(2S)-1,1,1-trifluoropropan-2-yl 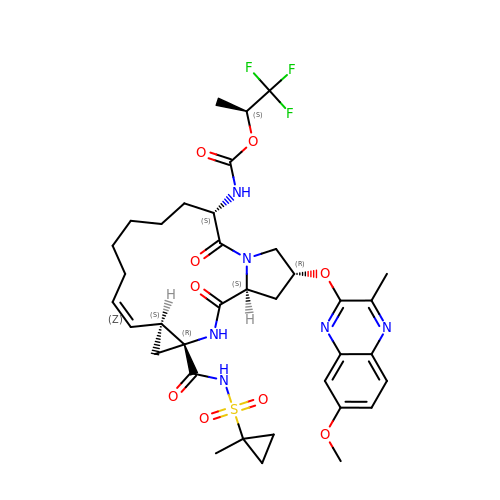{(2R,4S,6S,12Z,13aS,14aR,16aS)-2-[(7-methoxy-3-methylquinoxalin-2-yl)oxy]-14a-[(1-methylcyclopropane-1-sulfonyl)carbamoyl]-5,16-dioxo-1,2,3,5,6,7,8,9,10,11,13a,14,14a,15,16,16a-hexadecahydrocyclopropa[e]pyrrolo[1,2-a][1,4]diazacyclopentadecin-6-yl}carbamate | C36 H45 F3 N6 O9 S | RTCPQVJDZHADDP-NOIRXTOFSA-N>MASVSSATFSGHGARSLLQFLRLVGQLKRVPRTGWVYRNVQRPESVSDHMYRMAVMAMVIKDDRLNKDRCVRLALVHDMAECIVGDIAPADNIPKEEKHRREEEAMKQITQLLPEDLRKELYELWEEYETQSSAEAKFVKQLDQCEMILQASEYEDLEHKPGRLQDFYDSTAGKFNHPEIVQLVSELEAERSTNIAAAA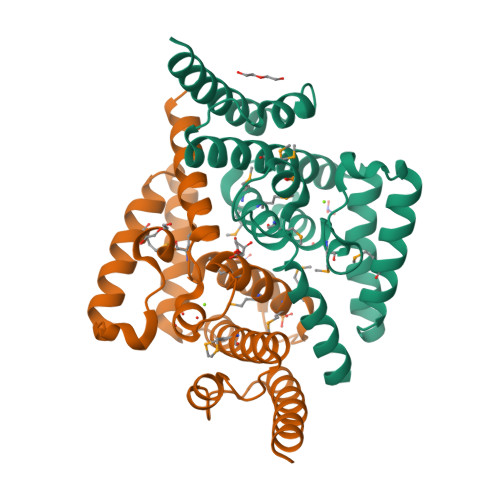SEPHS[2x]> C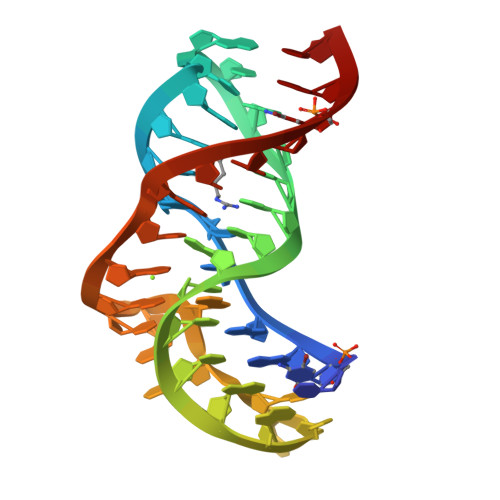CGGACGAGGUGCGCCGUACCCGGUCAGGACAAGACGGCGC;> CCGGACGAGGUGCGCCGUACCCGGUCACGACAAGACGGCGC>[2x]MRVLGIETSCDETGIAIYDDEKGLLANQLYSQVKLHADYGGVVPELASRDHVRKTVPLIQAALKESGLTAKDIDAVAYTAGPGLEGALLVGATVGRSLAFAWDVPAIPVHHMEGHLLAPMLEDNPPEFPFVALLVSGGHTQLISVTGIGQYELLGESIDDAAGEAFDKTAKLLGLDYPGGPLLSKMAAQGTAGRFVFPRPMTDRPGLDFSFSGLKTFAANTIRDNGTDDQTRADIARAFEDAVVDTLMIKCKRALDQTGFKRLVMAGGVSANRTLRAKLAEMMKKRRGEVFYARPEFCTDNGAMI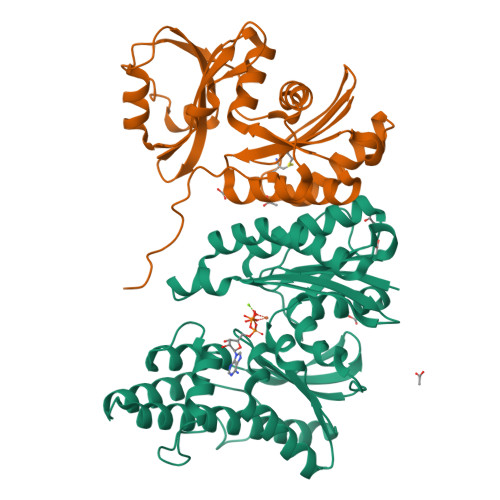AYAGMVRFKAGATADLGVSVRPRWPLAELPAAHHHHHH;>[2x]MRILAIDTATEACSVALWNDGTVNAHFELCPREHTQRILPMVQDILTTSGTSLTDINALAYGRGPGSFTGVRIGIGIAQGLALGAELPMIGVSTLMTMAQGAWRKNGATRVLAAIDARMGEVYWAEYQRDENGIWHGEETEAVLKPEIVHERMQQLSGEWVTVGTGWQAWPDLGKESGLVLRDGEVLLPAAEDMLPIACQMFAEGKTVAVEHAEPVYLRNNVAWKKLPGKEHHHHHH>TLPKRVKIVEVGPRDGLQNEKNIVSTPVKIKLIDMLSEAGLSVIETTSFVSPKWVPQMGDHTEVLKGIQKFPGINYPVLTPNLKGFEAAVAAGAKEVVIFGAASELFTKKNINCSIEESFQR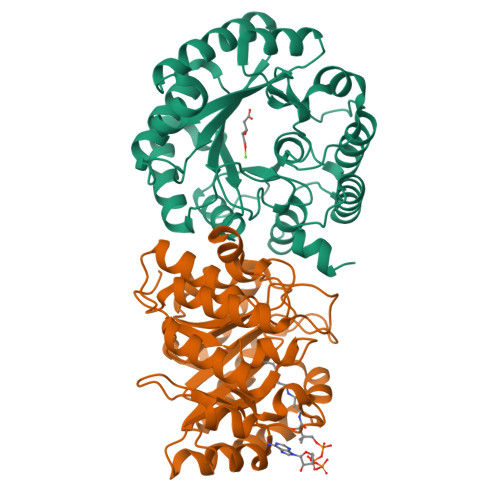FDAILKAAQSANISVRGYVSCALGCPYEGKISPAKVAEVTKKFYSMGCYEISLGDTIGVGTPGIMKDMLSAVMQEVPLAALAVHCHDTYGQALANTLMALQMGVSVVDSSVAGLGGCPYAQGASGNLATEDLVYMLEGLGIHTGVNLQKLLEAGNFICQALNRKTSSKVAQATCKL[6x]> MAEVTYKGKSFEVDEDGFLLRFDDWCPEWVEYVKESEGISDISPDHQKIIDFLQDYYKKNGIAPMVRILSKNTGFKLKEVYELFPSG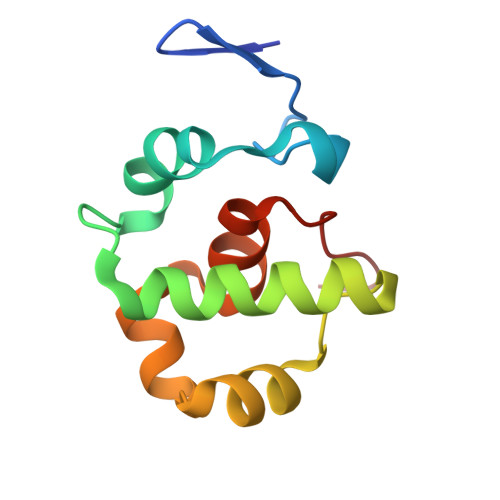PGKGACKMAGLPKPTGCV> MNVSIEEFTHFDFQLVPEPSPLDLVITEPLKNHIEVNGVKSGALLPLPFQTGIGKTYTALNFLLQQMLEQVRSELKEENTGKKSKRLLYYVTDSVDNVVSAKADLLKLIEKQTVKGEPRFTLEQQEYLKAQIVHLPNQSEQLLQCSDAVLNDVLIGFNLNAERDVQAEWSAISGLRRHASNPEVKISLNRQAGYFYRNLIDRLQKKQKGADRVLLSGSLLASVETLLPGEKIRNGSAHVAFLTTSKFLKGFHNTRSRYSPLRDLSGAVLIIDEIDKQNQVILSELCKQQAQDLIWAIRTLRANFRDHQLESSPRYDKIEDLFEPLRERLEEFGTNWNLAFAFNTEGANLNERPVRLFSDRSFTHVSSATHKLSLKSDFLRRKNLIFSDEKVEGSLIEKHGLLTRFVNEADVIYQWFLGTMRKAVFQYWENVRGLEIEVRENRSLEGTFQEAVQSLLTHFNLQEFESAVYESFDTRGLRQSAGGKANKLSSSKSYHHTGLKLVEVAHNQGTRDTVNCKASFLNTSPSGVLADMVDAGAVILGISATARADTVIHNFDFKYLNERLGNKLLSLSREQKQRVNNYYHSRRNYKDNGVVLTVKYLNSRDAFLDALLEEYKPEARSSHFILNHYLGIAESEQAFVRSWLSKLLASIKAFISSPDNRYMLSLLNRTLDTTRQNINDFIQFCCDKWAKEFNVKTKTFFGVNADWMRLVGYDEISKHLNTELGKVVVFSTYASMGAGKNPDYAVNLALEGESLISVADVTYSTQLRSDIDSIYLEKPTQLLLSDDYSHTANQLCQFHQILSLQENGELSPKSAENWCRQQLMGMSRERSLQQYHQTSDYQSAVRKYIEQAVGRAGRTSLKRKQILLFVDSGLKEILAEESRDPSLFSHEYVALVNKAKSAGKSIVEDRAVRRLFNLAQRNNKDGMLSIKALVHRLHNQPASKSDIQEWQDIRTQLLRYPTVAFQPERFNRLYLQSMTKGYYRYQGNLDGDPNSFEFFDRVPYGDMVSEEDCSLATLVQNQYVRPWFERKGFACSWQKEANVMTPIMFTNIYKGALGEQAVEAVLTAFDFTFEEVPNSIYERFDNRVIFAGIEQPIWLDSKYWKHEGNESSEGYSSKIALVEEEFGPSKFIYVNALGDTSKPIRYLNSCFVETS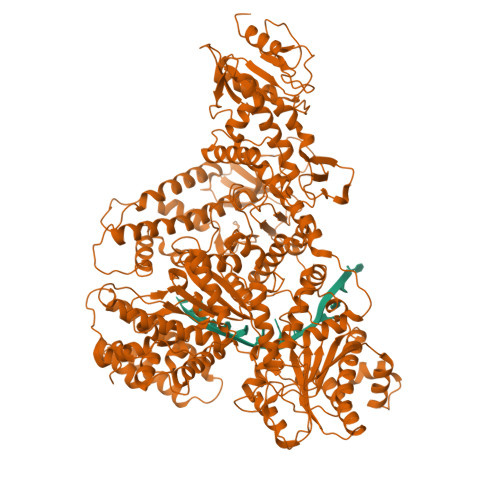PQLAKVIEIPALIDDSNADTNRTAVQELIKWLHHS>LVSSPSTLNPGTNVAKLAEQAPVHWVSVAQIENSLTGRPPMAVGFDIDDTVLFSSPGFWRGKKTYSPDSDDYLKNPAFWEKMNNGWDEFSIPKEAARQLIDMHVRRGDSIYFVTGRSQTKTETVSKTLADNFH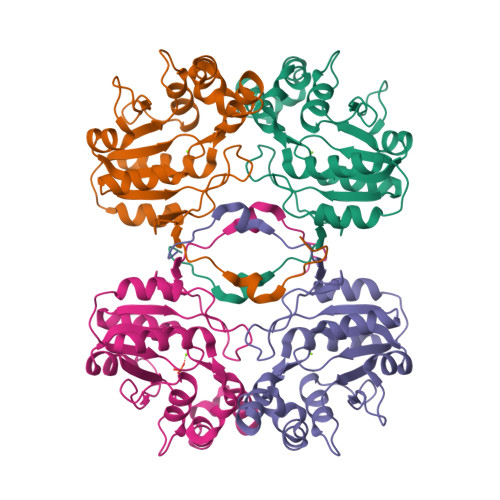IPAANMNPVIFAGDKPEQNTKVQWLQEKNMRIFYGDSDNDITAARDCGIRGIRILRAANSTYKPLPQAGAFGEEVIVNSEY[4x]>MQRARPGELVEVIMFRPTGKARVSNLDESMAMEFTDLRTRAMSSAAMIRQSVAAKTLLIENEDGKGSTRMEVQDFMKRFHMHASEDDKTGSPSTAWGTLRFPTKEATAPYLRLSVNDDPEDALLFVKAMLAQKYGETYDRPSLILSVTGGARNFTLPPRLETAIAKGLRLAAQRTNAWVVTGGTNTGVMKLTGQIMEALSKTQSHFIPPTIGIATYGVIIGGDDMTRGEPPKIGLEYEMHKKDPPKTTPLDDNHNLFLLVDDGSTNKFGKEIKFRAAFENAAGQAFAAPVVTIVVQGGPGTLGTALQAVRQGTPIVVVDGSGLAADVLAYAYNFMHNPLTRFKSYTIDDLRQKVAQTFNPKSSQQLTNLLDSALECVQDPNLVVVYSLQESGIDEFDDCILKAIFSSQGKLGNKLKQAMYFDQLDVAKRALSEASKNGQHNEIAACINDNLMAAMMHNKPHFVELYLGFDAKIYELKPSEEVAKTNITALDELPSFALAIEELYKREAKKPHSHVQRLVSLSNTDVLGRHYRVSTQRGDGTTRRIGRDLANTRAYNVLRMDQIFARLVSKDFSVNRDFTIYDSKYDKVPGIQFRRTAQASHMLFLWAICLDRFRMARHFWLIGDQSIINALVASRILERLSTHRALQGPHLAEERAKMQHNAKKFEELAVGVLGECHGSDSHMASEMLHSKNDMFNKKNAINIAYDAKSLAFLSHPATQSVINADWYGHLKSVTSFWAVLFAFFFPFFVLPFINFSEDHAEQQVEAPRDFFTDAPRSSHSANSTTSGAHRLRRKFAKFYSAPYTRFISDLLSHFVLCVVTSYFVLDKLEDTISAIEWILLVWFVALLLEELRQMIFCDGIAEYISDTWNRLDLIMITLFFVGFFTHASDPSNQDSKVVSKGIHAFLVVVLWLRFMRYYALSKNLGPKLIMMMEMMKDVSTFVFLLLIFLIGYGVAAQSLLSPDEDFSSRTFIGVLFRPYFQIYGELFLDDLNSEANCLGDTPFTECSRETVRMVPFFLAVYILGSNVLLVNLLIAMFNDTYMKVQEAAEDLWRKQNYELCAEYKDRPFLPAPFILLAHVHMLFMRLLRLCGVHTQEHEKIQDDETKRKITTFEELNTDKFLRRWERERQEMLEARVKMTNDNVVQAMGMMDQLLEHMISFRFSLDQQATKIKQEIRDDGLPSTEPTGLVSRTPSQPINRLNSAVAVHGHTAEAA[4x]

We investigated a TRPM2 chanzyme from choanoflagellates that integrates two seemingly incompatible functions into a single peptide: a channel module activated by ADP-ribose with high open probability and an enzyme module (NUDT9-H domain) consuming ADP-ribose at a remarkably slow rate. Using time-resolved cryogenic-electron microscopy, we captured a complete series of structural snapshots of gating and catalytic cycles, revealing the coupling mechanism between channel gating and enzymatic activity. The slow kinetics of the NUDT9-H enzyme module confers a self-regulatory mechanism: ADPR binding triggers NUDT9-H tetramerization, promoting channel opening, while subsequent hydrolysis reduces local ADPR, inducing channel closure. The structures of srTRPM2 exhibit a characteristic TRPM architecture, from top to bottom, a transmembrane domain (TMD) layer containing the ion-conducting pore, a signal transduction layer consisting of MHR3/4 domain and the C-terminal rib helix, and an ADPR-sensing layer consisting of the N-terminal MHR1/2 domain and the C-terminal NUDT9-H domain.

The tetramerization of the NUDT9-H domain through the buckle helix remodels the interface between the enzymatic module and the channel module. This raises the question of whether the NUDT9-H enzyme module plays a direct role in channel gating of srTRPM2 on ADPR binding. To this end, we generated a truncated construct by removing NUDT9-H, srTRPM2–ΔNUDT9-H. Despite reduced protein expression level at the plasma membrane, the truncation construct still responded to ADPR and Ca2+, generating currents with similar characteristics to the WT. This is distinct to human TRPM2 (hsTRPM2), in which removal of NUDT9-H abolished ADPR-induced current. Single-channel analysis of srTRPM2–ΔNUDT9-H revealed channel gating kinetics similar to the WT, albeit with a reduced open rate. Notably, this construct exhibited long-lived closed states between bursts of channel opening, a pattern not observed in the WT protein. In agreement with the functional data, the overall structure of srTRPM2–ΔNUDT9-H closely resembles the channel module of srTRPM2, but with some minor conformational changes that may have contributed to the subtle differences in gating kinetics. Our result indicates that the NUDT9-H domain is dispensable for the channel activation of srTRPM2, which is consistent with the nvTRPM2 chanzyme, but plays a role in the regulation of the channel activity.> MPVLLGIPLLLRFLGFLLVTLFGYLLTFLKKGFGKIAIAISLFLALIIGLNSILVGYLSDISAQLPSDFVQGVQLILPSNALPCFYVILSVKAAIF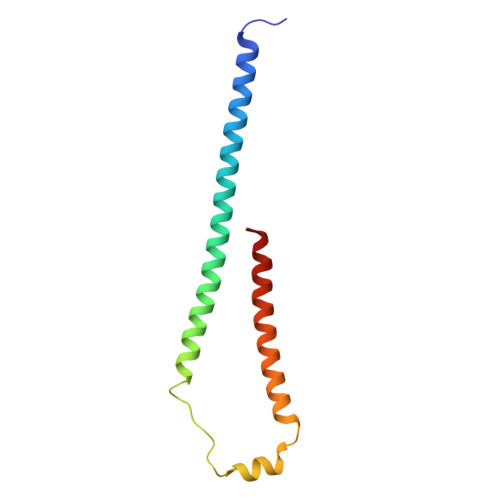IFDVKQKIVSYLDWDK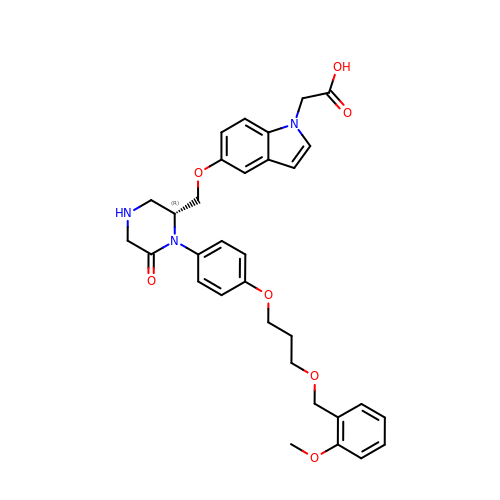(5-{[(2R)-1-(4-{3-[(2-METHOXYBENZYL)OXY]PROPOXY}PHENYL)-6-OXOPIPERAZIN-2-YL]METHOXY}-1H-INDOL-1-YL)ACETIC ACID | C32 H35 N3 O7 | VWRBPASGKKTVFT-AREMUKBSSA-N>MVLERNETMYYGGSLWSPPSNWNPFTPWNAVPGTTGLVYETMFFYDPLTGNFDPWLAEKGEWLDSKTYRVVLREGIYWHDNVPLTSEDVRFTFEIAKKYKGIHYSSVWEWLDHIETPDNRTVIFVFKDPRYHEWNELLYTLPIVPKHIWEEKDETTILQSSNEYPLGSGPYVAHSWDQNKMIFERFENWWGTKVMGVKPAPKYVVIVRVLSNNVALGMLMKGELDFSNFMLPGVPILKKVYNLNTWYDEPPYHLSSTVVGLFLNARKYPLSLPEFRRAIAMSINADPIVQRVYEGAVLKADPLGFLPNSVWMKYYPKE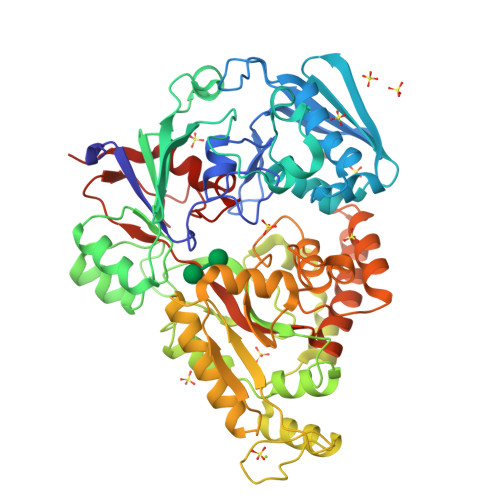VVEKHGFKYDPEEAKSILDKLGFRDVNGDGFRETPDGKPIKLTIECPYGWTDWMQAIQVIVDQLKVVGINAEPYFPDSSKYYENMYKGEFDIEMNANGTGISSTPWTYFNTIFYPDALESEFSYTGNYGRYQNPEVESLLEELNRTPLDNVEKVTELCGKLGEILLKDLPFIPLWYGAMAFITQDNVWTNWPNEHNPYAWPCGWANWWQTGALKILFNLKPAKHHHHHH[2x]> GSHMVLKFPKQQLPPKKKRRVGTTVHCDYLNRPHKSIHRRRTDPMVTLSSILESIINDMRDLPNTYPFHTPVNAKV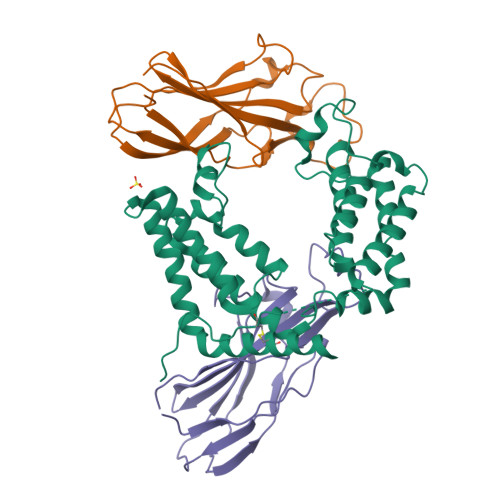VKDYYKIITRPMDLQTLRENVRKRLYPSREEFREHLELIVKNSATYNGPKHSLTQISQSMLDLCDEKLKEKEDKLARLEKAINPLLDDDDQVAFSFILDNIVTQKMMAVPDSWPFHHPVNKKFVPDYYKVIVNPMDLETIRKNISKHKYQSRESFLDDVNLILANSVKYNGPESQYTKTAQEIVNVCYQTLTEYDEHLTQLEKDICTAKEAALEEA;>[2x]GSHMAKVQVNNVVVLDNPSPFYNPFQFEITFECIEDLSEDLEWKIIYVGSAESEEYDQVLDSVLVGPVPAGRHMFVFQADAPNPGLIPDADAVGVTVVLITCTYRGQEFIRVGYYVNNEYTETELRENPPVKPDFSKLQRNILASNPRVTRFHINWED>[2x]GMTLPPYHTPLPAETLRALSIPAPWTFGLADRVRFGELDAIGHVNHTAYLRWYESFRLPFLKARHVTDYGPTSPRLVLKQVHCTYLAEMGMGEDYVITGRVSNFRTTSFTME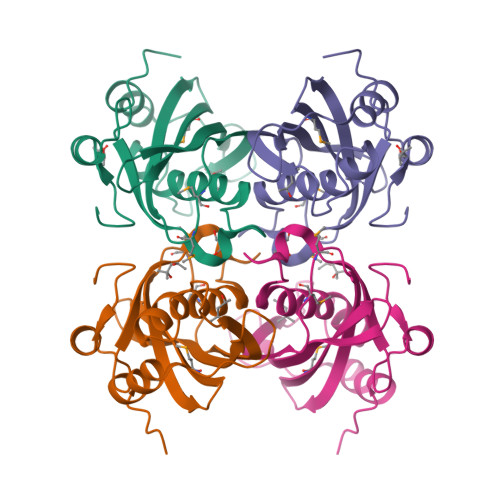FACWRLGDAVECTSEGSAVVVLLNRDGSGRYPIPEAGRASFVTEDGVLAAG> MSSPDFSAGRELRTQGARIAGVVSCVPSKQVDNDYFVERFDASAVRDVVKMIGVNRRRWADAQTSAGDLCRKAGEKLLAGLGWQADSIDALIFVSQTPNYRLPATAFVLQAELDLPASCLALDINLGCSGYPQALWLGMNLIQTGAAKRVLLAVGDTISKMIDPTDRSTSLLFGDAGTMTALETSNGDAAAHFIIGADGKGARNLIVPSGGFKPYDAAADERMAGKSPECLFMDGGEIFNFTLNAVPKLVSRTLDIAGRDKDSYDAFLFHQANLFMLKHLAKKAGLPAERVPVNIGEYGNTSCASIPLLITTELKDRLKEETLQLGMFGFGVGYSWASAALAVGPLNIVDTIET

Here we report a functional and structural genomics effort that applied saturation-level transposon mutagenesis and next generation sequencing (Tn-seq) to identify essential genes in B. thailandensis, followed by high-throughput structure determination. We used an “ortholog rescue” approach to maximize structural coverage of these gene families, which are likely to be essential not only in B. thailandensis, but also in related, but more virulent, Burkholderia species, such as B. pseudomallei. Using only seven Burkholderia species to select orthologs of essential genes, we solved structures for 49/406 essential gene families, and for 56 total Burkholderia protein targets (including seven ortholog replicates). Of these 56 targets, 25 satisfied criteria for being a potential antimicrobial drug target.

By using an ortholog rescue strategy for insoluble or difficult to crystallize targets, we increased our structural coverage of B. thailandensis essential genes from 31/406 (7.6%) to 49/406 (12.1%). Ortholog structures may also be useful in designing broad-spectrum antibiotics with cross-species activity, and by representing a variety of functionally conservative point mutations in the active site may be useful in developing drugs less susceptible to mutations that cause drug resistance.>MANKFKTLDKMVYNLLLEKIKNGELVPNEHLAEEKLAREFGVSRSPLRKAIATLTAQGIVSYHENSGAVLNDCIVDADRYVQLMETIEIFVDAA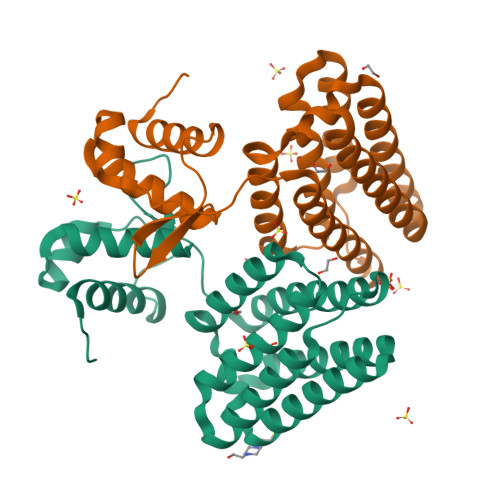IAKAAHFGYEMDLEKLYARMQEMERFSYLTDLENYFDAHHRFILCLISFAENPYQVRIVKQIFFQMVHFSDGINMFKSVEIREWTNKKSNQIYELLAEGKIELARKTIKSMFAELTIQAYRLEHHHHHH[2x]> MGSSHHHHHHGSMYGVYRAMKLPIYLDYSATTPVDPRVAEKMMQFMTMDGTFGNPASRSHRFGWQAEEAVDIARNQIADLVGADPREIVFTSGATESDNLAIKGAANFYQKKGKHIITSKTEHKAVLDTCRQLEREGFEVTYLAPQRNGIIDLKELEAAMRDDT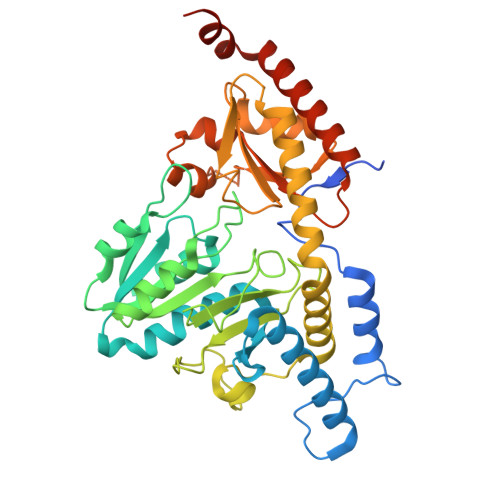ILVSIMHVNNEIGVVQDIAAIGEMCRARGIIYHVDATQSVGKLPIDLSQLKVDLMSFSGHKIYGPKGIGALYVRRKPRVRIEAQMHGGGHERGMRSGTLPVHQIVGMGEAYRIAKEEMATEMERLRGLRNRLWNGIKDIEEVYLNGDLEHGAPNILNVSFNYVEGESLIMALKDLAVSSGSACTSASLEPSYVLRALGLNDELAHSSIRFSLGRFTTEEEIDYTIELVRKSIGRLRDLSPLWEMYKQGVDLNSIEWAHH[(2S,4S)-4-{4-[1-phenyl-3-(trifluoromethyl)-1H-pyrazol-5-yl]piperidin-1-yl}pyrrolidin-2-yl](1,3-thiazolidin-3-yl)methanone 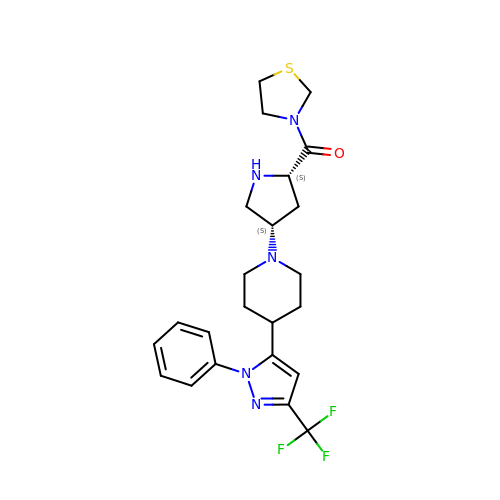| C23 H28 F3 N5 O S | CYNIHEXFNGMKLP-OALUTQOASA-N>APSFDCGKPQVEPKKCPGRVVGGCVAHPHSWPWQVSLRTRFGMHFCGGTLISPEWVLT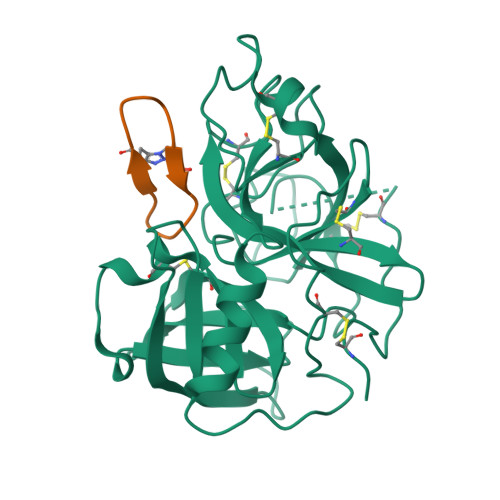AAHCLEKSPRPSSYKVILGAHQEVNLEPHVQEIEVSRLFLEPTRKDIALLKLSSPAVITDKVIPACLPSPNYVVADRTECFITGWGETQGTFGAGLLKEAQLPVIENKVCNRYEFLNGRVQSTELCAGHLAGGTDSCQGDSGGPLVCFEKDKYILQGVTSWGLGCARPNKPGVYVRVSRFVTWIEGVMRNN[2x];>[2x]GRAYKSKPPIAFPD> ASCETTVTSGDTMTYSTRSISVPASCAE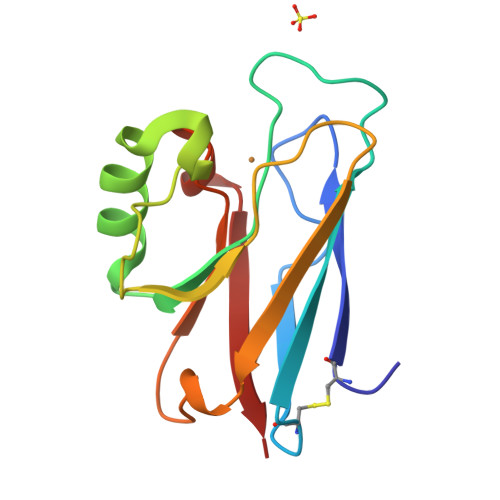FTVNFEHKGHMPKTGMGHNWVLAKSADVGDVAKEGAHAGADNNFVTPGDKRVIAFTPIIGGGEKTSVKFKVSALSKDEAYTYFCSYPGHFSMMRGTLKLEE> GDQLTHVVEEVKTYDLVWRSIKNLWEDVQRTFETPWCRVDVLLLQSDLANFLRRADELPRAVKQFEMYKSLFSQVNMLTSVNKILVELKDGALKPRHWNMIFRDIGKRQIQKNLLDKLEFSLKDVMVLNLTLNEILLTKIIERAQKEFVIEKSLNRIKKFWKEAQYEVIEHSSGLKLVREWDVLEQACKEDLEELVSMKASNYYKIFEQDCLDLESKLTKLSEIQVNWVEVQFYWLDLYGILGENLDIQNFLPLETSKFKSLTSEYKMITTRAFQLDTTIEVIHIPNFDTTLKLTIDSLKMIKSSLSTFLERQRRQFPRFYFLGNDDLLKIIGSGKHHDQVSKFMKKMFGSIESIIFFEDSITGVRSVEGEVLNLNEKIELKDSIQAQEWLNILDTEIKLSVFTQFRDCLGQLKDGTDIEVVVSKYIFQAILLSAQVMWTELVEKCLQTNEFSKYWKEVDMKIKGLLDKLNKSSDNVKKKIEALLVEYLHFNNVIGQLKNCSTKEEARLLWAKVQKFYQKNDTLDDLNSVFISQSGYLLQYKFEYIGIPERLIYTPLLLVGFATLTDSLHQKYGGCFFGPAGTGKTETVKAFGQNLGRVVVVFNCDDSFDYQVLSRLLVGITQIGAWGCFDEFNRLDEKVLSAVSANIQQIQNGLQVGKSHITLLEEETPLSPHTAVFITLNPGYNGRSELPENLKKSFREFSMKSPQSGTIAEMILQIMGFEDSKSLASKIVHFLELLSSKCSSMNHYHFGLRTLKGVLRNCSPLVSEFGEGEKTVVESLKRVILPSLGDTDELVFKDELSKIFDSAGTPLNSKAIVQCLKDAGQRSGFSMSEEFLKKCMQFYYMQKTQQALILVGKAGCGKTATWKTVIDAMAIFDGHANVVYVIDTKVLTKESLYGSMLKATLEWRDGLFTSILRRVNDDITGTFKNSRIWVVFDSDLDPEYVEAMNSVLDDNKILTLPNGERLPIPPNFRILFETDNLDHTTPATITRCGLLWFSTDVCSISSKIDHLLNKSYEALDNKLSMFELDKLKDLISDSFDMASLTNIFTCSNDLVHILGVRTFNKLETAVQLAVHLISSYRQWFQNLDDKSLKDVITLLIKRSLLYALAGDSTGESQRAFIQTINTYFGHDSQELSDYSTIVIANDKLSFSSFCSEIPSVSLEAHEVMRPDIVIPTIDTIKHEKIFYDLLNSKRGIILCGPPGSGKTMIMNNALRNSSLYDVVGINFSKDTTTEHILSALHRHTNYVTTSKGLTLLPKSDIKNLVLFCDEINLPKLDKYGSQNVVLFLRQLMEKQGFWKTPENKWVTIERIHIVGACNPPTDPGRIPMSERFTRHAAILYLGYPSGKSLSQIYEIYYKAIFKLVPEFRSYTEPFARASVHLYNECKARYSTGLQSHYLFSPRELTRLVRGVYTAINTGPRQTLRSLIRLWAYEAWRIFADRLVGVKEKNSFEQLLYETVDKYLPNQDLGNISSTSLLFSGLLSLDFKEVNKTDLVNFIEERFKTFCDEELEVPMVIHESMVDHILRIDRALKQVQGHMMLIGASRTGKTILTRFVAWLNGLKIVQPKIHRHSNLSDFDMILKKAISDCSLKESRTCLIIDESNILETAFLERMNTLLANADIPDLFQGEEYDKLLNNLRNKTRSLGLLLDTEQELYDWFVGEIAKNLHVVFTICDPTNNKSSAMISSPALFNRCIINWMGDWDTKTMSQVANNMVDVVPMEFTDFIVPEVNKELVFTEPIQTIRDAVVNILIHFDRNFYQKMKVGVNPRSPGYFIDGLRALVKLVTAKYQDLQENQRFVNVGLEKLNESVLKVNELNKTLSKKSTELTEKEKEARSTLDKMLMEQNESERKQEATEEIKKILKVQEEDIRKRKEVVMKSIQDIEPTILEAQRGVKNIKKQQLTEIRSMVNPPSGVKIVMEAVCAILGYQFSNWRDIQQFIRKDDFIHNIVHYDTTLHMKPQIRKYMEEEFLSDPNFTYETINRASKACGPLYQWVNAQINFSKVLENVDPLRQEMKRIEFESLKTKANLLAAEEMTQDLEASIEVSKQKYSLLIRDVEAIKTEMSNVQANLDRSISLVKSLTFEKERWLNTTKQFSKTSQELIGNCIISSIYETYFGHLNERERGDMLVILKRLLGKFAVKYDVNYRFIDYLVTLDEKMKWLECGLDKNDYFLENMSIVMNSQDAVPFLLDPSSHMITVISNYYGNKTVLLSFLEEGFVKRLENAVRFGSVVIIQDGEFFDPIISRLISREFNHAGNRVTVEIGDHEVDVSGDFKLFIHSCDPSGDIPIFLRSRVRLVHFVTNKESIETRIFDITLTEENAEMQRKREDLIKLNTEYRLKLKNLEKRLLEELNNSQGNMLENDELMVTLNNLKKEAMNIEKKLSESEEFFPQFDNLVEEYSIIGKHSVKIFSMLEKFGQFHWFYGISIGQFLSCFKRVFIKKSRETRAARTRVDEILWLLYQEVYCQFSTALDKKFKMIMAMTMFCLYKFDIESEQYKEAVLTMIGVLSESSDGVPKLTVDTNDDLRYLWDYVTTKSYISALNWFKNEFFVDEWNIADVVANSENNYFTMASERDVDGTFKLIELAKASKESLKIIPLGSIENLNYAQEEISKSKIEGGWILLQNIQMSLSWVKTYLHKHVEETKAAEEHEKFKMFMTCHLTGDKLPAPLLQRTDRVVYEDIPGILDTVKDLWGSQFFTGKISGVWSVYCTFLLSWFHALITARTRLVPHGFSKKYYFNDCDFQFASVYLENVLATNSTNNIPWAQVRDHIATIVYGGKIDEEKDLEVVAKLCAHVFCGSDNLQIVPGVRIPQPLLQQSEEEERARLTAILSNTIEPADSLSSWLQLPRESILDYERLQAKEVASSTEQLLQEM

Cytoplasmic dynein-1 (dynein) is a highly conserved molecular motor that moves toward the microtubule minus end, transporting various cargoes including RNAs, membrane vesicles, and viruses, and plays a crucial role in cell division. Dynein belongs to the ATPase associated with various cellular activities (AAA+) family of proteins. Its heavy chain features a motor domain composed of six AAA+ modules, a long stalk, a microtubule-binding domain (MTBD) located at the end of the stalk, a buttress region that makes additional connections between the AAA5 module and the stalk, and a long tail that interacts with dynactin and an activating adapter. Lis1 is a dimer (~90 kDa) with an amino-terminal dimerization domain and carboxy-terminal β-propellers that bind to the dynein motor domain24,25. Our data support a model in which Lis1 relieves dynein autoinhibition by increasing its basal ATP hydrolysis rate and promoting conformations compatible with complex assembly and motility.

We purified wild-type yeast dynein monomer (amino acids 1352–4092) in the absence of any nucleotide, plunge-froze grids after the addition of excess ATP (500-fold) at two time points (0.5 min and 30 min) incubating the samples at 4 °C to slow nucleotide hydrolysis. We grouped the reconstructions into three distinct conformations on the basis of the position of dynein’s linker, a mechanical element that adopts different conformations in response to the ATP-hydrolysis-driven opening and closing of the ring: ‘straight’ (yellow outline), ‘interm’ (intermediate, green outline), and ‘bent’ (blue outline). To understand how ATP hydrolysis affects dynein structurally, we built models of different high-resolution dynein conformations identified in our datasets. We mapped nucleotides to their binding pockets, as all our structures showed nucleotide densities in the AAA modules. Although our maps have only partial densities in the stalk region, the ring opening and the stalk’s CC1 and CC2 positions in dynein with a straight linker is consistent with a strong microtubule-binding state, as indicated by the lack of bulging of CC2 in the stalk region characteristic of the weak microtubule-binding state. The intermediate linker dynein has partial density that fits a model in which the CC2 has a slight bulge in the stalk and is consistent with a semi-bent, also called semi-α state that could represent an intermediate microtubule binding state. In our dataset, the comparison of the straight and intermediate linker dynein shows movement in the AAA domains, even though the nucleotide states are the same in these structures. In the straight and intermediate dynein state, when Lis1 is not bound to dynein, the linker interacts with the AAA2 H2 loop, but these contact sites are less resolved when Lis1 is bound, suggesting reduced engagement in this region.Some bacteriophage encode a recombinase that catalyzes single-stranded DNA annealing (SSA). Redβ belongs to a large group of proteins annotated as the RecT family based on the protein from the rac prophage of E. coli. Here, we have used single-particle cryo-EM to determine a 3.4 Å structure of a homolog of λ-Redβ from the A118 prophage of Listeria innocua that we will refer to as LiRecT. The structure confirms that the RecT/Redβ family of annealing proteins share a common core fold with RAD52.

To determine if there is a similar structural transition for LiRecT, we prepared a complex of it with just one 83-mer ssDNA and obtained a ~5 Å resolution cryo-EM reconstruction by single particle analysis. Surprisingly, the LiRecT-ssDNA complex also exists as left-handed helical filaments, instead of as rings, but they are not as well ordered, and they do not stack end-to-end. Using a monomer of LiRecT from the complex with annealed duplex, 8 subunits of LiRecT could be docked into the reconstruction for the central portion of the filament. Due to the lower resolution of this reconstruction, we could not fit the ssDNA to the map, although there is strong density for DNA in the groove above α2 and α3. Strikingly, the density for the portion of each LiRecT subunit at the upper rim of the filament is almost completely absent in the structure with ssDNA, for the entire length of the filament. This upper N-terminal lobe of each monomer (N-lobe), which is formed by the αA–αC bundle and the β1–β2 hairpin, would likely clamp down on the DNA once the second strand is incorporated, to form the additional protein-DNA and inter-subunit interactions that are shown in Fig. 4 for the complex with annealed duplex. Moreover, cryo-EM images collected for LiRecT protein without DNA reveal smaller particles that are much less well ordered, suggesting that the filament is assembled on the ssDNA (a full data set without DNA was not collected).

>[8x]GSHMATNDELKNQLANKQNGGQVASAQSLDLKGLLEAPTMRKKFEKVLDKKAPQFLTSLLNLYNGDDYLQKTDPMTVVTSAMVAATLDLPIDKNLGYAWIVPYKGRAQFQLGYKGYIQLALRTGQYKSINVIEVREGELLKWNRLTEEIELDLDNNTSEKVVGYCGYFQLINGFEKTVYWTRKEIEAHKQKFSKSDFGWKKDYDAMAKKTVLRNMLSKWGILSIDMQTAVTEDEAEPRERKDVTDDESIPDIIDAPVTPSDTLEAGSVVQGSMI1-[4-(piperidin-1-ylsulfonyl)phenyl]-3-(pyridin-3-ylmethyl)thiourea | C18 H22 N4 O2 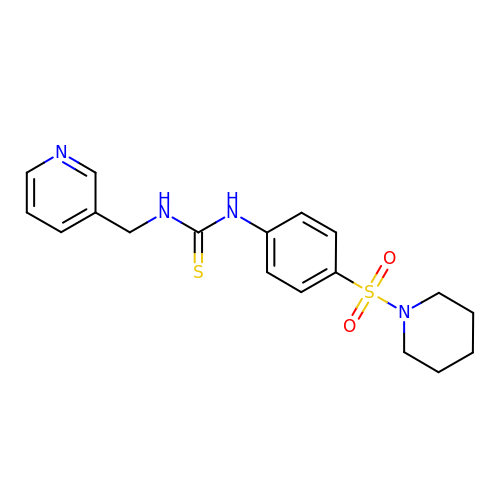S2 | NIADLWNDYLCGNO-UHFFFAOYSA-N4-[[3,5-bis(fluoranyl)phenyl]carbonylamino]-~{N}-piperidin-4-yl-1~{H}-pyrazole-3-carboxamide 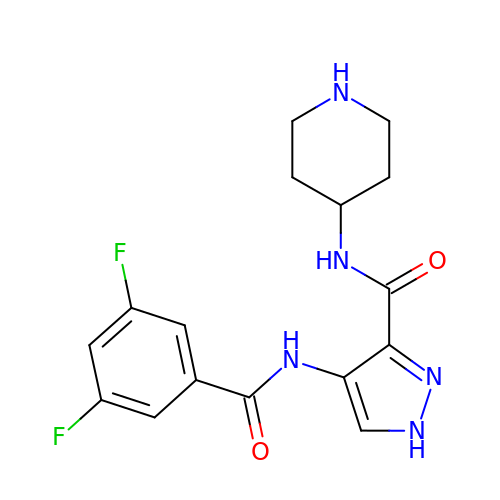| C16 H17 F2 N5 O2 | NIHAFOURWLZLFN-UHFFFAOYSA-N> MEIERINEHTVKFYMSYGDIEDRGFDREEIWYNRERSEELFWEVMDEVHEEEEFAVEGPLWIQVQALDKGLEIIVTKAQLSKDGQKLELPIPEDKKQEPASEDLDALLDDFQKEEQAVNQEEKEQKLQFVLRFGDFEDVISLSKLNVNGSKTTLYSFENRYYLYVDFCNMTDEEVENQLSILLEYA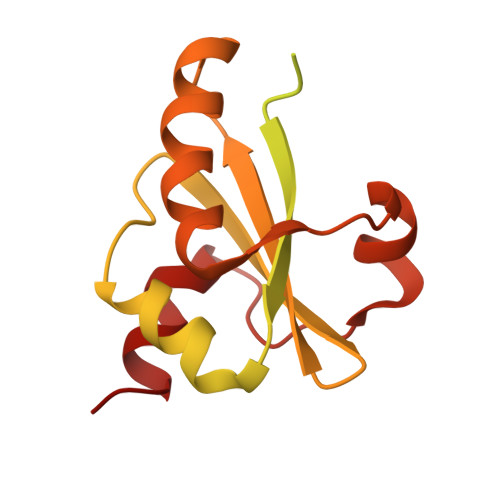TESSISIHRLEEYGKLIISEHALETIKKHFAS> MQEEPTNIPRPDNAELLVASEVAIENAAIALSEIVSVVNTSDGRIEVFGVGTDNAVWHN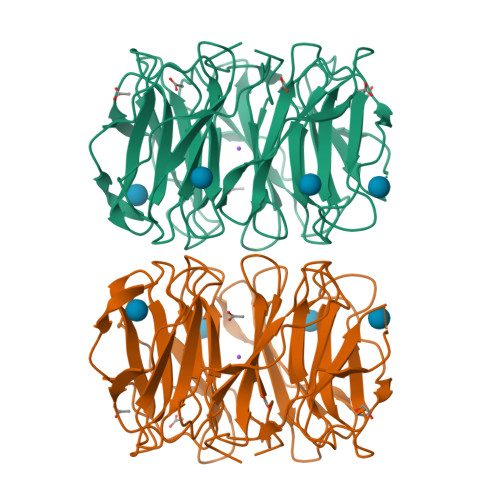RQTAPHSGSSWTGWISLNGKVTSKPVVYINTDGRLEVFARGTDNALWHIWQTATNAGWSNWQSLGGTITSNPAVYVNTDGRIDVFARGTDNALWHISQTAAHSGPWSSWQSLNGVITSNPAVHINSDGRLEVFARGTDNALWHIWQTAPDSNQWSGWDSLGGVITSDPVVIGTADGRLEVFARGSNNALYHIWQTVPHGGPWSNWASLNGVITSAPAVVKNSDGRLEVFARGTNNALYHIWQTVSHSGPWSNWATLNGTITSAPTAVEDADGRLEVFARGTDNALWNIWQATPSWSAWVSLKGSLIDASAIK(6R)-6-(4-methoxyphenyl)-2-methyl-6-(3-pyrimidin-5-ylphenyl)pyrrolo[3,4-d][1,3]thiazol-4-amine 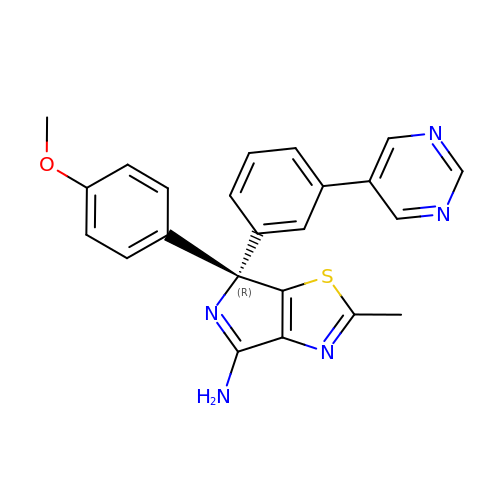| C23 H19 N5 O S | YQFNSFOVYAQJAF-HSZRJFAPSA-N> SLSAHEIRELFLSFFEKKGHTRVKSAPLVPENDPTLLFVNAGMVPFKNVFLGLEKRPYKRATSCQKCLRVSGKHNDLEQVGYTSRHHTFFEMLGNFSFGDYFKKEAIEYAWEFVTEVLKLPKEKLYVSVYKDDEEAYRIWNEHIGIPSERIWRLGEEDNFWQMGDVGPCGPSSEIYVDRGEEYEGDERYLEIWNLVFMQYNRDENGVLTPLPHPNIDTGMGLERIASVLQGKNSNFEIDIIFPLIQFGEEVSGKKYGEKFETDVALRVIADHLRAITFAISDGVIPSNEGRGYVIRRILRRAMRFGYKLGIEN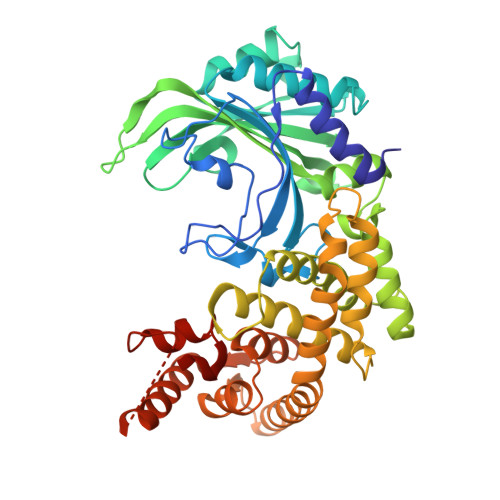PFLYKGVDLVVDIMKEPYPELELSREFVKGIVKGEEKRFIKTLKAGMEYIQEVIQKALEEGRKTLSGKEVFTAYDTYGFPVDLIDEIAREKGLGIDLEGFQCELEEQRERARKHFKVEAKKVKPVYSHLKELGKTSAFVGAAALEHHHHHH> HGTNFLKDHRFGSYAAIQENALAKWYVNAKGYFEDVANAMEEANEEIFITDWWLSPEIFLKRPVVEGNRWRLDCILKRKAQQGVRIFIMLYKEVELALGINSEYTKRTLMRLHPNIKVMRHPDHVSSTVYLWAHHEKLVIIDQSVAFVGGIDLAYGRWDDNEHRLTDVGSVFWHGKDYCNFVFKDWVQLDKPFADFIDRYSTPRMPWHDIASAVHGKAARDVARHFIQRWNFTKIMKSKYRSLSYPFLLPKSQTTAHELRYQVPGSVHANVQLLRSAADWSAGIKYHEESIHAAYVHVIENSRHYIYIENQFFISCADDKVVFNKIGDAIAQRILKAHRENQKYRVYVVIPLLPGFEGDISTGGGNALQAIMHFNYRTMCRGENS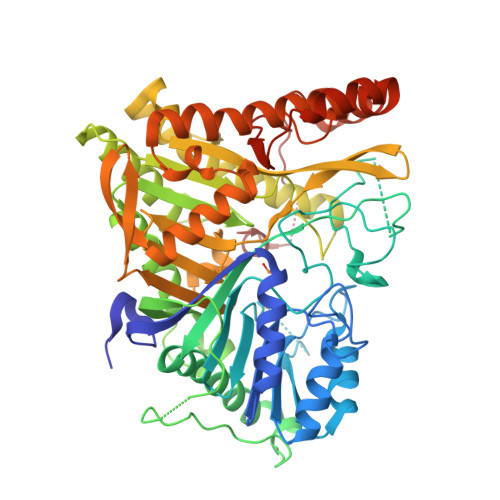ILGQLKAELGNQWINYISFCGLRTHAELEGNLVTELIYVHSKLLIADDNTVIIGSANINDRSMLGKRDSEMAVIVQDTETVPSVMDGKEYQAGRFARGLRLQCFRVVLGYLDDPSEDIQDPVSDKFFKEVWVSTAARNATIYDKVFRCLPNDEVHNLIQLRDFINKPVLAKEDPIRAEEELKKIRGFLVQFPFYFLSEESLLPSVGTKEAIVPMEVWT N-[(1r,4r)-4-{3-[5-amino-3-(4-sulfamoylanilino)-1H-1,2,4-triazole-1-carbonyl]-2,4-difluorophenyl}cyclohexyl]prop-2-enamide | C24 H25 F2 N7 O4 S | 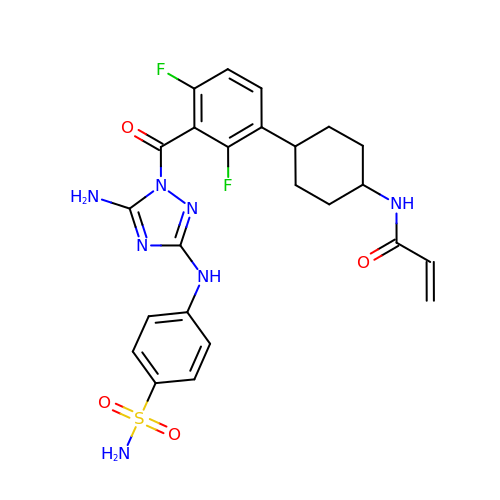VCGXFVJENSAIDN-HDJSIYSDSA-N> SDLPMPMRFRHLKKTSKEAVGVYRSPIHGRGLFCKRNIDAGEMVIEYAGIVIRSILTDKREKYYDSKGIGSSYMFRIDDSEVVDATMHGNAARFINHSCEPNCYSRVINIDGQKHIVIFAM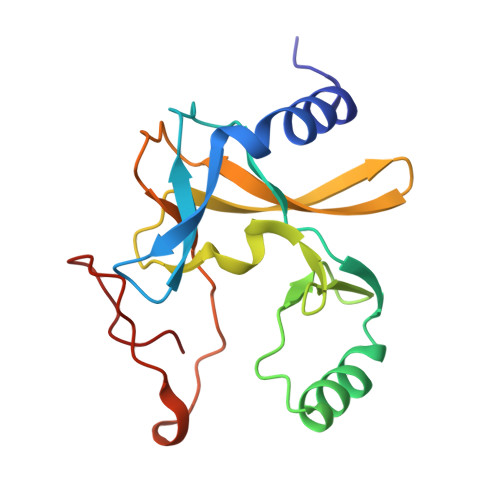RKIYRGEELTYDYKFPIEDASNKLPCNCGAKKCRKFLN SULFITE ION | O3 S | 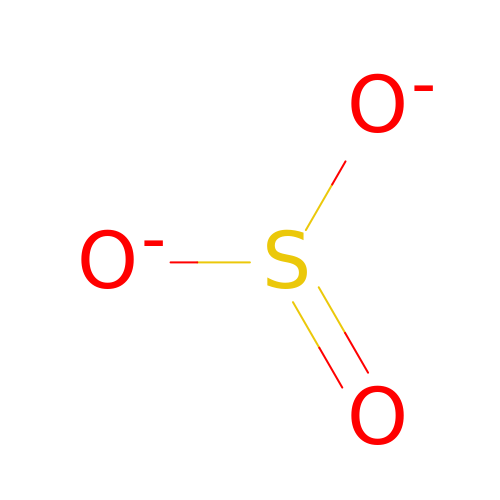LSNNMFCWUKXFEE-UHFFFAOYSA-L> EAPHLVQVDAARALWPLRRFWRSTGFCPPLPHSQADPYVLSWDQQLNLAYVGAVPHRGIKQVRTHWLLELVTTRGSTGQGLSYNFTHLDGYLDLLRENQLLPGFELMGSASGHFTDFEDKQQVFEWKDLVSSLARRYIGRYGLAHVSKWNFETWNEPDHHDFDNVSMTMQGFLN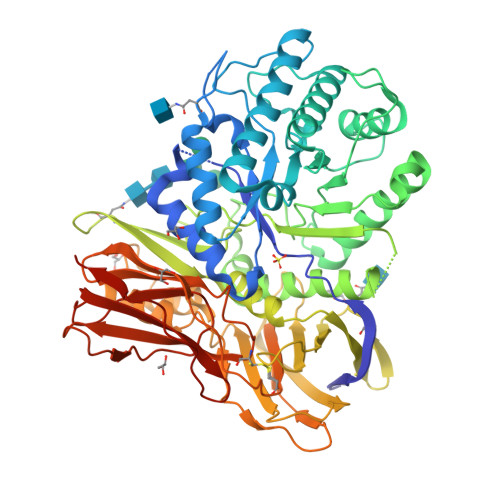YYDACSEGLRAASPALRLGGPGDSFHTPPRSPLSWGLLRHCHDGTNFFTGEAGVRLDYISLHRKGARSSISILEQEKVVAQQIRQLFPKFADTPIYNDEADPLVGWSLPQPWRADVTYAAMVVKVIAQHQNLLLANTTSAFPYALLSNDNAFLSYHPHPFAQRTLTARFQVNNTRPPHVQLLRKPVLTAMGLLALLDEEQLWAEVSQAGTVLDSNHTVGVLASAHRPQGPADAWRAAVLIYASDDTRAHPNRSVAVTLRLRGVPPGPGLVYVTRYLDNGLCSPDGEWRRLGRPVFPTAEQFRRMRAAEDPVAAAPRPLPAGGRLTLRPALRLPSLLLVHVCARPEKPPGQVTRLRALPLTQGQLVLVWSDEHVGSKCLWTYEIQFSQDGKAYTPVSRKPSTFNLFVFSPDTGAVSGSYRVRALDYWARPGPFSDPVPYLEVPVPRGPPSPGNP>[4x]MGHHHHHHSSPKIEERTYPPQIPAQQELGDFSAYQSVLPEPLRKAEKLLQETGIKE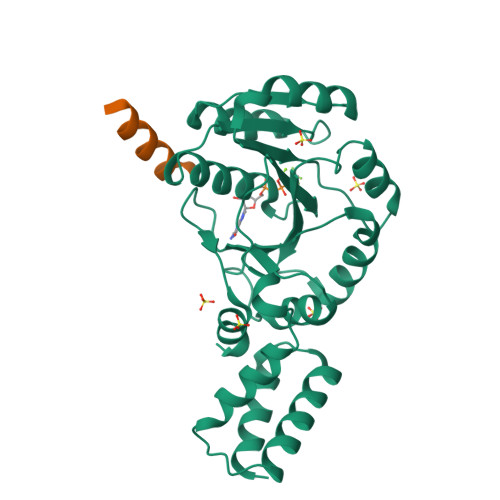STKTNTLKKLLRFSVEAGGLTEENVVGKLQEILCDMLPSADKWQEPIHSKYIVLFGSTGAGKTTTLAKLAAISMLEKHKKIAFITTDTYRIAAVEQLKTYAELLQAPLEVCYTKEEFQQAKELFSEYDHVFVDTAGRNFKDPQYIDELKETIPFESSIQSFLVLSATAKYEDMKHIVKRFSSVPVNQYIFTKIDETTSLGSVFNILAESKIGVGFMTNGQNVPEDIQTVSPLGFVRMLCR;>[4x]MQMNRYDQAATLRAKMEKRERVL>[4x]HFLCGVVEGFYGRPWVMEQRKELFRRLQKWELNTYLYAPKDDYKHRMFWREMYSVEEAEQLMTLISAAREYEIEFIYAISPGLDITFSNPKEVSTLKRKLDQVSQFGCRSFALLFDNIDHNMCAADKEVFSSFAHAQVSITNEIYQYLGEPETFLFCPTEYCGTFCYPNVSQSPYLRTVGEKLLPGIEVLWTGPKVVSKEIPVESIEEVSKIIKRAPVIWDNIHANDYDQKRLFLGPYKGRSTELIPRLKGVLTNPNCEFEANYVAI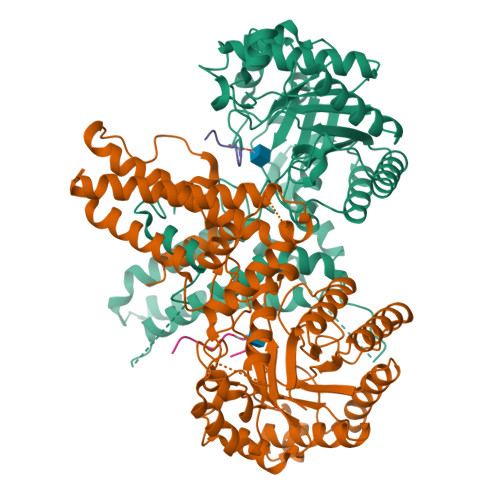HTLATWYKSNMNGVRKDVVMTDSEDSTVSIQIKLENEGSDEDIETDVLYSPQMALKLALTEWLQEFGVPHQYSSRGGGGSGGGGSVTLEDLQLLADLFYLPYEHGPKGAQMLREFQWLRANSSVVSVNCKGKDSEKIEEWRSRAAKFEEMCGLVMGMFTRLSNCANRTILYDMYSYVWDIKSIMSMVKSFVQWLGCRSHSSAQFLIGDQEPWAFRGGLAGEFQRLLPIDGANDLFFQ;>QLWVDSTPPPG[4x]The last two steps in this pathway occur through the activity of penicillin-binding proteins (PBPs). Class A PBPs perform both a glycosyltransferase activity (GTase), which polymerizes the lipid activated precursor molecules into a growing PG strand, and a d,d-transpeptidase activity, which catalyses the cleavage of a d-Ala4-d-Ala5 peptide bond of the acyl donor and subsequently crosslinks the d-Ala4 carbonyl to the primary amine of a diaminopimelic acid (DAP) residue on the acceptor (in Gram negatives such as Escherichia coli), resulting in a d-Ala4donor-DAP3acceptor crosslink. Inhibition of either of these crucial, PBP-mediated, final steps in PG biosynthesis results in destabilization of the cell wall and ultimately cell death. In all, the modelled regions span residues 82–98, 100–207, 212–236, 267–297, 286–542, and 547–798. The overall tri-partite architecture of PBP1b is as previously observed in MoeA-liganded structures, with the canonical and well-described C-terminal transpeptidase (TPase) domain, central putative activator binding domain (UB2H domain), and N-terminal membrane-anchored glycosyltransferase (GTase) domain all able to be modelled into the cryoEM reconstruction as a complete structure of the apo state of E. coli PBP1b.

Here, we determine the near-atomic resolution structure of the 83 kDa class A PBP from E. coli, PBP1b, using cryogenic electron microscopy (cryoEM) and a membrane mimetic. Following complete processing of the PBP1b data, including subtraction by masking of clear features corresponding to the SMA membrane mimetic in initial maps, a cryoEM reconstruction of the apo state of E. coli PBP1b was produced, showing well-resolved map features for all three domains of PBP1b and an overall resolution of 3.28 Å. Both before and after particle subtraction, the transmembrane helix was only observed where it packs against the GTase domain. Despite the expected broad structural conservation of the apo PBP1b in comparison to previously solved MoeA-liganded structures, significant domain rearrangements are observed between the two states. The TPase domain and the UB2H remain as a near-fixed domain dyad, but with an ~40° relative rotation of the GTase domain with respect to the fixed TPase/UB2H pair (measured by UCSF Chimera11). In comparison to MoeA-liganded structures of PBP1b, we propose that the observed ~40° relative rotation is likely ligand-induced. Most notable are conserved hydrogen bonds at the interface of the UB2H and TPase domains, including those between the side chain guanidino group of R109 and carboxylic acid of D443 (R109-D443) and the interaction between the backbone amide nitrogen of R109 and backbone carbonyl oxygen of F422 (R109-F442). In the apo form, R134 adopts an extended rotamer conformation, with its guanidino group forming hydrogen bond interactions to both the carboxylic acid group of D345 and the backbone carbonyl of P398 (R134-D345 and R134-P398).

> KPRGKRGWLWLLLKLAIVFAVLIAIYGVYLDQKIRSRIDGKVWQLPAAVYGRMVNLEPDMTISKNEMVKLLEATQYRQVSKMTRPGEFTVQANSIEMIRRPFDFPDSKEGQVRARLTFDGDHLATIVNMENNRQFGFFRLDPRLITMISSPNGEQRLFVPRSGFPDLLVDTLLATEDRHFYEHDGISLYSIGRAVLANLTAGRTVQGASTLTQQLVKNLFLSSERSYWRKANEAYMALIMDARYSKDRILELYMNEVYLGQSGDNEIRGFPLASLYYFGRPVEELSLDQQALLVGMVKGASIYNPWRNPKLALERRNLVLRLLQQQQIIDQELYDMLSARPLGVQPRGGVISPQPAFMQLVRQELQAKLGDKVKDLSGVKIFTTFDSVAQDAAEKAAVEGIPALKKQRKLSDLETAIVVVDRFSGEVRAMVGGSEPQFAGYNRAMQARRSIGSLAKPATYLTALSQPKIYRLNTWIADAPIALRQPNGQVWSPQNDDRRYSESGRVMLVDALTRSMNVPTVNLGMALGLPAVTETWIKLGVPKDQLHPVPAMLLGALNLTPIEVAQAFQTIASGGNRAPLSALRSVIAEDGKVLYQSFPQAERAVPAQAAYLTLWTMQQVVQRGTGRQLGAKYPNLHLAGKTGTTNNNVDTWFAGIDGSTVTITWVGRDNNQPTKLYGASGAMSIYQRYLANQTPTPLNLVPPEDIADMGVDYDGNFVCSGGMRILPVWTSDPQSLCQQSEMQQQPS>[2x]GAMTKPRFTTGLVYDTLMLKHQCTAGSSSSHPEHAGRIQSIWSRLQETGLRGKCEAIRGRKATLEELQTVHSEAHTLLYGTNPLNRQKLDSKKLLGSLASVFVRLPCGGVGVDSDTIWNEVHS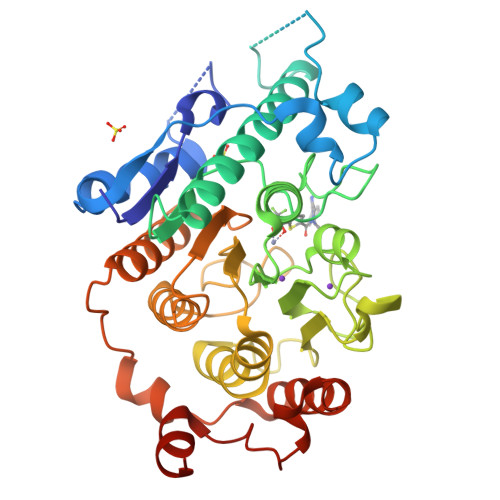AGAARLAVGCVVELVFKVATGELKNGFAVVRPPGHHAEESTPMGFCYFNSVAVAAKLLQQRLSVSKILIVDWDVHHGNGTQQAFYSDPSVLYMSLHRYDDGNFFPGSGAPDEVGTGPGVGFNVNMAFTGGLDPPMGDAEYLAAFRTVVMPIASEFAPDVVLVSSGFDAVEGHPTPLGGYNLSARCFGYLTKQLMGLAGGRIVLALEGGHDLTAICDASEACVSALLGNELDPLPEKVLQQRPNANAVRSMEKVMEIHSKYWRCLQRTTSTAGRSLIEAQTCENEEAETVT> MHHHHHHSSGRENLYFQGMRYVIMQSRDIRENLATEDYLLNTLSFEE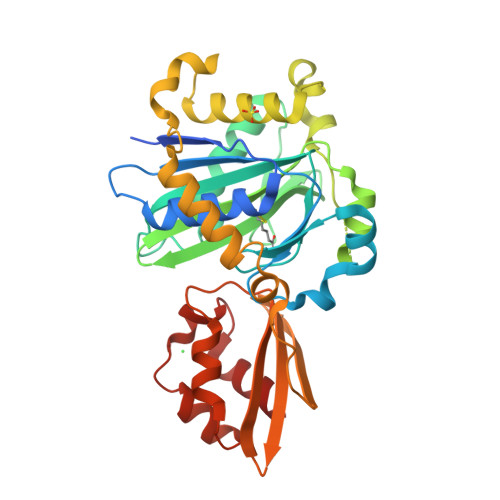PLVLFYIQEPCVILGRNQNAYEEIDLAYAREKGIVITRRLSGGGAVYDDLGNVSFSFVVQEGHQAFGDFKAFTKPIIEALHKMGATGAEISGRNDLLIDGKKFSGNAMYTKKGKMYTHGTLMYDVDLAEVQRVLTVSKKKIESKGTKSVRGRVTNLRPYLDEKYQQLTIEEFRNRLLMELFDVESLTEIAEKEYVLTKADQQEIRKLVAEVYGNEAWIFGEAPKFTIKKEEKFKGGIVDARLTVEKGKIIELTIYGDYFAKKETTEIVAALLGVDYQYSSIWQALAAFNFEDYFVNITKEEFVHLLVD propan-2-yl dodecanoate 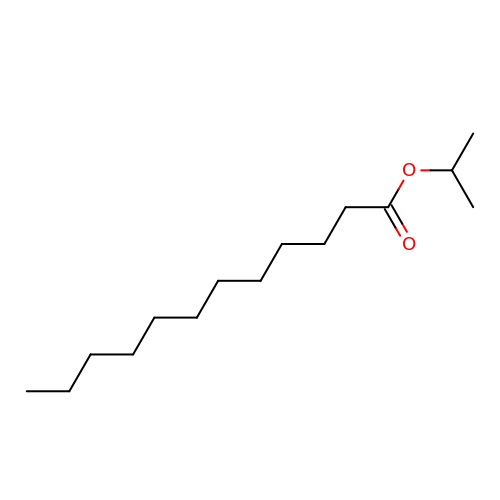| C15 H30 O2 | UJPPXNXOEVDSRW-UHFFFAOYSA-N5'-O-[(R)-{[(2S)-2-aminopropanoyl]oxy}(hydroxy)phosphoryl]adenosine 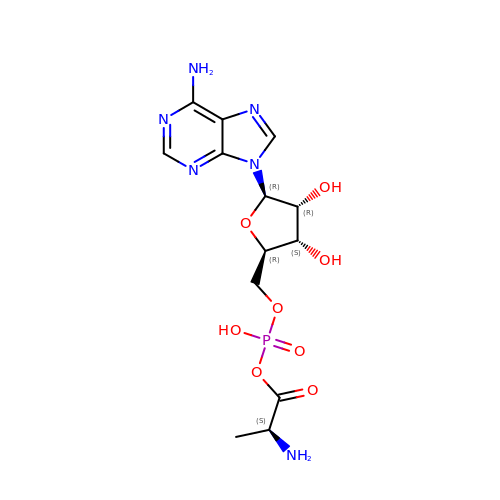| C13 H19 N6 O8 P | ISYFCRWDMNBLTM-MACXSXHHSA-N>[20x]M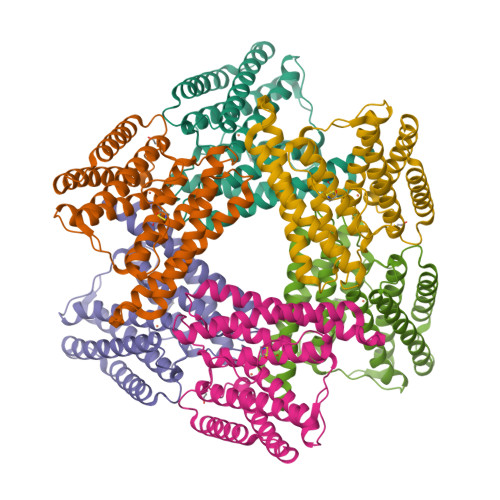SLERNYEESALFEHQFWLKVLTDHAQFLLDALAPKEKEDIKKATYFVETFTNLLNKVRNVNLMAFSKEAEQAAKEIRAFKLNIIQKQLEGKITIHFTPTFINHMVNEVEEYIAVLEFLKKGEVPPVFHELHYHLVWLTDAAGHAGSISGGLDLVEKRLKEKSEEFTKHFEQFYLKAVEMTGYLRTELHHFPALKKFTKDVSLELKLFSHFLHEVEELELSNEVLSVLSARMADHMAREECYYLLKLAQSSGLEMPKCNPLEGHHHHHH> MSDGAVQPDGGQPAVRNERATGSGNGSGGGGGGGSGGVGISTGTFNNQTEFKFLENGWVYITANSSRLVHLNMPESENYRRVVVNNLDKTAVNGNMALDDTHAEIVTPWSLVDANAWGVWFNPGDWQLIVNTMSELHLVSFEQEIFNVVLKTVSESATQPPTKVYNNDLTASLMVALDSNNTMPFTPAAMRSETLGFYPWKPTIPTPWRYYFQWDRTLIPSHTGTSGTPTNIYHGTDPDDVQFYTIENSVPVHLLRTGDEFATGTFFFDCKPCRLTHTWQTNRALGLPPFLNSLPQSEGGTNFGYIGVQQDKRRGVTQMGNTNYITEATIMRPAEVGYSAPYYSFEASTQGPFKTPIAAGRGGAQTDENQAADGDPRYAFGRQHGQKTTTTGETPERFTYIAHQDTGRYPEGDWIQNINFNLPVTDDNVLLPTDPIGGKTGINYTNIFNTYGPLTALNNVPPVYPNGQIWDKEFDTDLKPRLHVNAPFVCQNNCPGQLFVKVAPNLTNQYDPDASANMSRIVTYSDF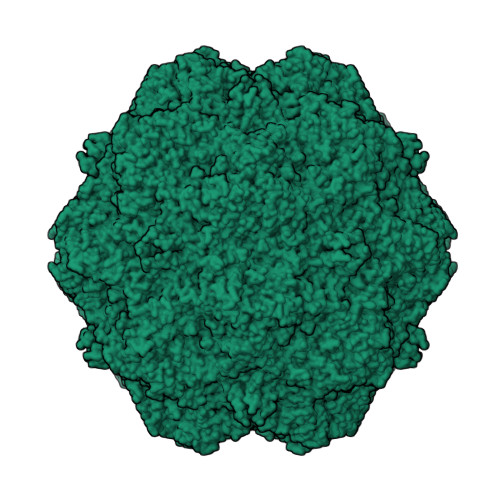WWKGKLVFKAKLRASHTWNPIQQMSINVDNQFNYVPSNIGGMKIVYEKSQLAPRKLY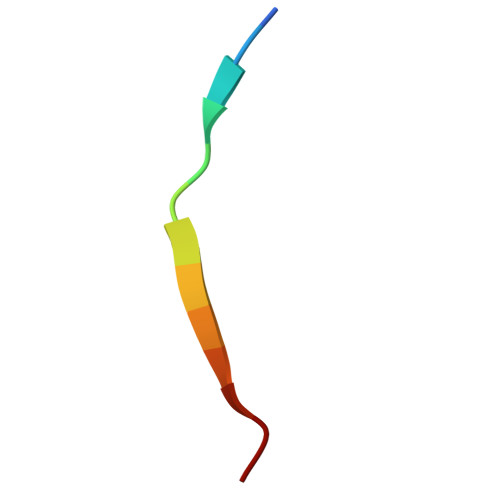> AAAAFVLFMAAAA> GPMATVFRQENVDDYYDTGEELGSGQFAVVKKCREKSTGLQYAAKFIKKRRTKSSRRGVSREDIEREVSILKEIQHPNVITLHEVYENKTDVILILELVAGGELFDFLAEKESLTEEEATEFLKQILNGVYYLHSLQIAHFDLKPENIMLLDRNVPKPRIKIIDFGLAHKIDFGNEFKNIFGTPEFVAPEIVNYEPLGLEADMWSIGVITYILL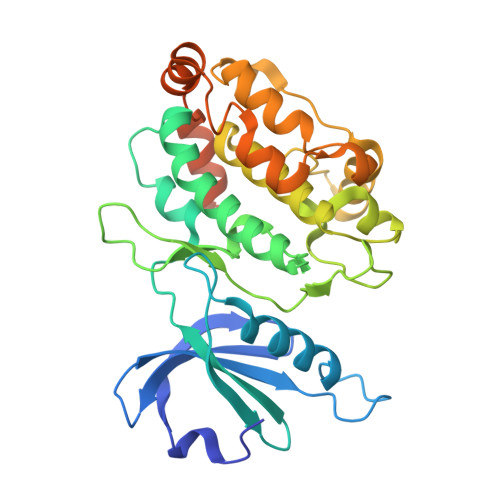SGASPFLGDTKQETLANVSAVNYEFEDEYFSNTSALAKDFIRRLLVKDPKKRMTIQDSLQHPWIKPKDTQQALSRKAAAVNMEKFKKFAARKKWKQAVRLISLCQRLSRSFLSRSNMSVARSD>MPVRRGHVAPQNTFLDTIIRKFEGQSRKFIIANARVENCAVIYCNDGFCELCGYSRAEVMQRPCTCDFLHGPRTQRRAAAQIAQALLGAEERKVEIAFYRKDGSCFLCLVDVVPVKNEDGAVIMFILNFEVVMEKDMVGSSPTSDREIIAPKIKERTHNVTEKVTQVLSLGADVLPEYKLQAPRIHRWTILHYSPFKAVWDWLILLLVIYTAVFTPYSAAFLLKETEEGPPATECGYACQPLAVVDLIVDIMFIVDILINFRTTYVNANEEVVSHPGRIAVHYFKGWFLIDMVAAIPFDLLIFGSGSEELIGLLKTARLLRLVRVARKLDRYSEYGAAVLFLLMCTFALIAHWLACIWYAIGNMEQPHMDSRIGWLHNLGDQIGKPYNSSGLGGPSIKDKYVTALYFTFSSLTSVGFGNVSPNTNSEKIFSICVMLIGSLMYASIFGNVSAIIQRLYSGTARYHTQMLRVREFIRFHQIPNPLRQRLEEYFQHAWSYTNGIDMNAVLKGFPECLQADICLHLNRSLLQHCKPFRGATKGCLRALAMKFKTTHAPPGDTLVHAGDLLT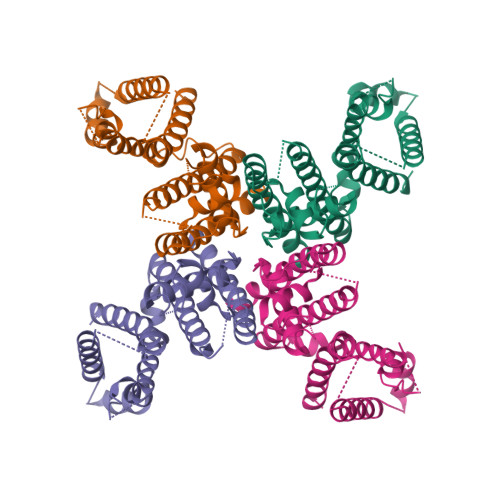ALYFISRGSIEILRGDVVVAILGKNDIFGEPLNLYARPGKSNGDVRALTYCDLHKIHRDDLLEVLDMYPEFSDHFWSSLEITFNLRDTNMIPGGRQYQELPRCPAPTPSLLNIPLSSPGRRPRGDVESRLDALQRQLNRLETRLSADMATVLQLLQRQMTLVPPAYSAVTTPGPGPTSTSPLLPVSPLPTLTLDSLSQVSQFMACEELPPGAPELPQEGPTRRLSLPGQLGALTSQPLHRHGSDPGSLEVLFQ[4x]> MDADSLLLSLELASGSGQGLSPDRRASLLTSLMLVKRDYRFARVLFWGRILGLVADYYIAQGLSEDQLAPRKTLYSLNCTEWSLLPPATEEMAMQISVVSGRFMGDPSHEYEHTELQKVNEGEKVFDEEVVVQIKEETRLVSIIDQIDKAVAIIPRGALFKTPFGVTHVNRTFEGLPLSEVRKLSSYFHFREAIDLKNKTLLEKSDLEPSLDFLDSLEYDIPRGSWSIQMER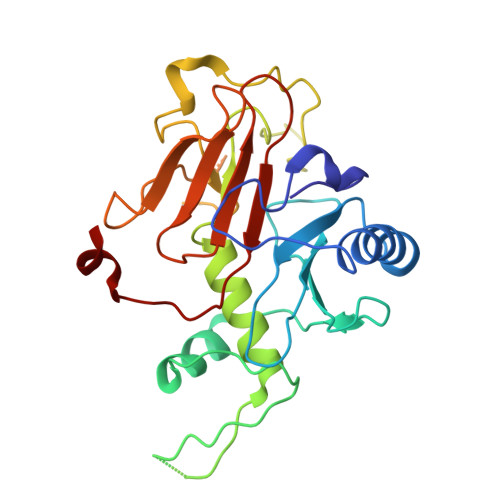GNALVVLRSLLWPGLTFYHAPRTKNYGYIYVGTGEKNMDLPFML> GSDSDFTFTLPAGRKECFYQPMPLKASLEIEYQVLDGGELDIDFHLTSPEGRTLVFEQRKSDGVHTIETEDGDYMFCFDNTFSTISEKVIF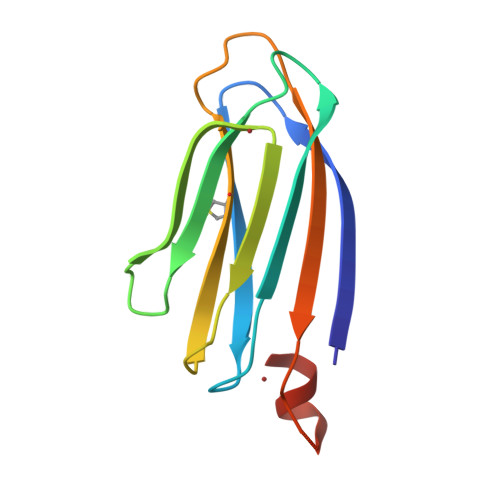FELILDNMGEEVQGQEDWKKYIT>[2x]MTTTATLTYPFHDWSQELSPRYAQLRASDAPVCPVVSEGTGDHLWLATRYAAAVELLEDPRLSSEAAIASGAPRQEPVELRAPGTRADGVAMLREAGLRSVLADGLGPRAV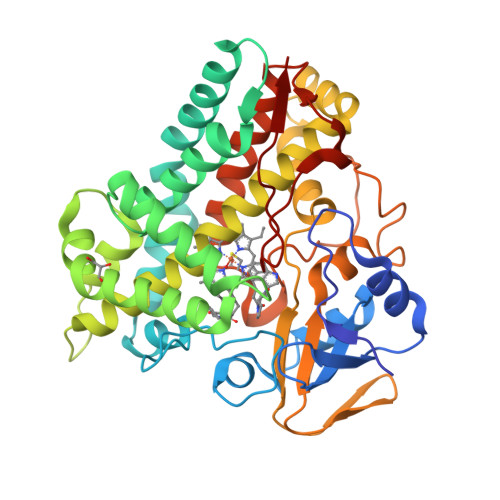RRHQGWINDLAETLMSALASREGTFDLAADFVEPLSSALVSRTLLGELSADERDLLAHCADTGLRFCGVTHEEQVHAFTQMHEFFLEHARRLAGTPGEHLLKLIAEAPVDHGPLSDEALAEAGSLLVVAGFPTSSGFLCGALLTLLRHPDAVQELHAHPERVPSAVEELLRYTPLSTGSVKRMATEDLEIDGVRIKVGEVVMVSLEAVNHDPDAFEDPDVFRPGREGPMHFGFGRGRHFCPGNRLARCVIEATVRAVARRPGLRLAVAPEEISWHEGLFFRRPRAIPATW>[2x]NADNYKNVINRTGAPQYMKDYDYDDHQRFNPFFDLGAWHGHLLPDGPNTMGGFPGVALLTEEYINFMASNFDRLTVWQDGKKVDFTLEAYSIPGALVQKLTAKDVQVEM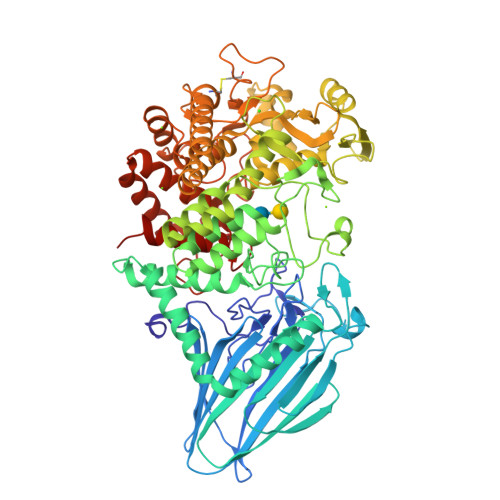TLRFATPRTSLLETKITSNKPLDLVWDGELLEKLEAKEGKPLSDKTIAGEYPDYQRKISATRDGLKVTFGKVRATWDLLTSGESEYQVHKSLPVQTEINGNRFTSKAHINGSTTLYTTYSHLLTAQEVSKEQMQIRDILARPAFYLTASQQRWEEYLKKGLTNPDATPEQTRVAVKAIETLNGNWRSPGGAVKFNTVTPSVTGRWFSGNQTWPWDTWKQAFAMAHFNPDIAKENIRAVFSWQIQPGDSVRPQDVGFVPDLIAWNLSPERGGDGGNWNERNTKPSLAAWSVMEVYNVTQDKTWVAEMYPKLVAYHDWWLRNRDHNGNGVPEYGATRDKAHNTESGEMLFTVKKGDKEETQSGLNNYARVVEKGQYDSLEIPAQVAASWESGRDDAAVFGFIDKEQLDKYVANGGKRSDWTVKFAENRSQDGTLLGYSLLQESVDQASYMYSDNHYLAEMATILGKPEEAKRYRQLAQQLADYINTCMFDPTTQFYYDVRIEDKPLANGCAGKPIVERGKGPEGWSPLFNGAATQANADAVVKVMLDPKEFNTFVPLGTAALTNPAFGADIYWRGRVWVDQFWFGLKGMERYGYRDDALKLADTFFRHAKGLTADGPIQANYNPLTGAQQGAPNFSWSAAHLYMLYNDFFRKQ> GNSIASCPEEQPHVGNYRLLRTIGKGNFAKVKLARHILTGREVAIKIIDKTQLNPSSLQKLFREVRIMKGLNHPNIVKLFEVIETEKTLYLVMEYASAGEVFDYLVSHGRMKEKEARAKFRQIVSAVHYCHQKNIVHRDLKAENLLLDAEANIKIADFGFSNEFTLGSKLDTFC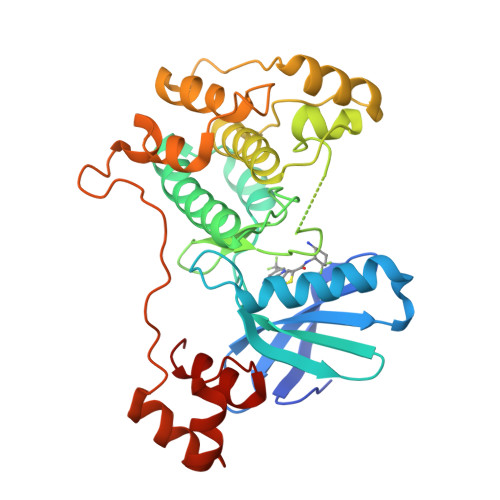GSPPYAAPELFQGKKYDGPEVDIWSLGVILYTLVSGSLPFDGHNLKELRERVLRGKYRVPFYMSTDCESILRRFLVLNPAKRCTLEQIMKDKWINIGYEGEELKPYTEPEEDFGDTKRIEVMVGMGYTREEIKESLTSQKYNEVTATYLLLGRK>[2x]MSDVAETLDPLRLPLQGERLIEASAGTGKTFTIAALYLRLLLGLGGSAAFPRPLTVEELLVVTFTEAATAELRGRIRSNIHELRIACLRETTDNPLYERLLEEIDDKAQAAQWLLLAERQMDEAAVFTIHGFCQRMLNLNAFESGMLFEQQLIEDESLLRYQACADFWRRHCYPLPREIAQVVFETWKGPQALLRDINRYLQGEAPVIKAPPPDDETLASRHAQIVARIDTVKQQWRDAVGELDALIESSGIDRRKFNRSNQAKWIDKISAWAEEETNSYQLPESLEKFSQRFLEDRTKAGGETPRHPLFEAIDQLLAEPLSIRDLVITRALAEIRETVAREKRRRGELGFDDMLSRLDSALRSESGEVLAAAIRTRFPVAMIDEFQDTDPQQYRIFRRIWHHQPETALLLIGDPKQAIYAFRGADIFTYMKARSEVHAHYTLDTNWRSAPGMVNSVNKLFSQTDDAFMFREIPFIPVKSAGKNQALRFVFKGETQPAMKMWLMEGESCGVGDYQSTMAQVCAAQIRDWLQAGQRGEALLMNGDDARPVRASDISVLVRSRQEAAQVRDALTLLEIPSVYLSNRDSVFETLEAQEMLWLLQAVMTPERENTLRSALATSMMGLNALDIETLNNDEHAWDVVVEEFDGYRQIWRKRGVMPMLRALMSARNIAENLLATAGGERRLTDILHISELLQEAGTQLESEHALVRWLSQHILEPDSNASSQQMRLESDKHLVQIVTIHKSKGLEYPLVWLPFITNFRVQEQAFYHDRHSFEAVLDLNAAPESVDLAEAERLAEDLRLLYVALTRSVWHCSLGVAPLVRRRGDKKGDTDVHQSALGRLLQKGEPQDAAGLRTCIEALCDDDIAWQTAQ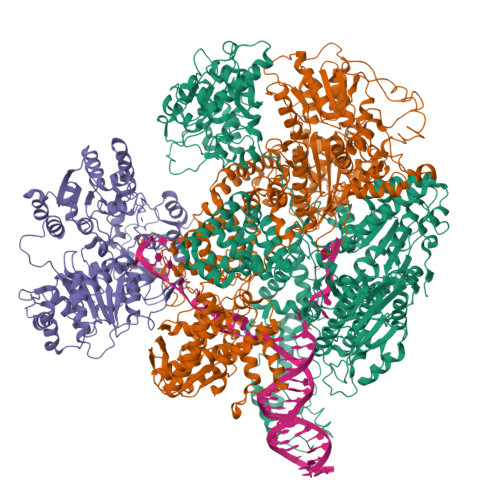TGDNQPWQVNDVSTAELNAKTLQRLPGDNWRVTSYSGLQQRGHGIAQDLMPRLDVDAAGVASVVEEPTLTPHQFPRGASPGTFLHSLFEDLDFTQPVDPNWVREKLELGGFESQWEPVLTEWITAVLQAPLNETGVSLSQLSARNKQVEMEFYLPISEPLIASQLDTLIRQFDPLSAGCPPLEFMQVRGMLKGFIDLVFRHEGRYYLLDYKSNWLGEDSSAYTQQAMAAAMQAHRYDLQYQLYTLALHRYLRHRIADYDYEHHFGGVIYLFLRGVDKEHPQQGIYTTRPNAGLIALMDEMFAGMTLEEA;>[2x]MLRVYHSNRLDVLEALMEFIVERERLDDPFEPEMILVQSTGMAQWLQMTLSQKFGIAANIDFPLPASFIWDMFVRVLPEIPKESAFNKQSMSWKLMTLLPQLLEREDFTLLRHYLTDDSDKRKLFQLSSKAADLFDQYLVYRPDWLAQWETGHLVEGLGEAQAWQAPLWKALVEYTHQLGQPRWHRANLYQRFIETLESATTCPPGLPSRVFICGISALPPVYLQALQALGKHIEIHLLFTNPCRYYWGDIKDPAYLAKLLTRQRRHSFEDRELPLFRDSENAGQLFNSDGEQDVGNPLLASWGKLGRDYIYLLSDLESSQELDAFVDVTPDNLLHNIQSDILELENRAVAGVNIEEFSRSDNKRPLDPLDSSITFHVCHSPQREVEVLHDRLLAMLEEDPTLTPRDIIVMVADIDSYSPFIQAVFGSAPADRYLPYAISDRRARQSHPVLEAFISLLSLPDSRFVSEDVLALLDVPVLAARFDITEEGLRYLRQWVNESGIRWGIDDDNVRELELPATGQHTWRFGLTRMLLGYAMESAQGEWQSVLPYDESSGLIAELVGHLASLLMQLNIWRRGLAQERPLEEWLPVCRDMLNAFFLPDAETEAAMTLIEQQWQAIIAEGLGAQYGDAVPLSLLRDELAQRLDQERISQRFLAGPVNICTLMPMRSIPFKVVCLLGMNDGVYPRQLAPLGFDLMSQKPKRGDRSRRDDDRYLFLEALISAQQKLYISYIGRSIQDNSERFPSVLVQELIDYIGQSHYLPGDEALNCDESEARVKAHLTCLHTRMPFDPQNYQPGERQSYAREWLPAASQAGKAHSEFVQPLPFTLPETVPLETLQRFWAHPVRAFFQMRLQVNFRTEDSEIPDTEPFILEGLSRYQINQQLLNALVEQDDAERLFRRFRAAGDLPYGAFGEIFWETQCQEMQQLADRVIACRQPGQSMEIDLACNGVQITGWLPQVQPDGLLRWRPSLLSVAQGMQLWLEHLVYCASGGNGESRLFLRKDGEWRFPPLAAEQALHYLSQLIEGYREGMSAPLLVLPESGGAWLKTCYDAQNDAMLDDDSTLQKARTKFLQAYEGNMMVRGEGDDIWYQRLWRQLTPETMEAIVEQSQRFLLPLFRFNQS;>[2x]MKLQKQLLEAVEHKQLRPLDVQFALTVAGDEHPAVTLAAALLSHDAGEGHVCLPLSRLENNEASHPLLATCVSEIGELQNWEECLLASQAVSRGDEPTPMILCGDRLYLNRMWCNERTVARFFNEVNHAIEVDEALLAQTLDKLFPVSDEINWQKVAAAVALTRRISVISGGPGTGKTTTVAKLLAALIQMADGERCRIRLAAPTGKAAARLTESLGKALRQLPLTDEQKKRIPEDASTLHRLLGAQPGSQRLRHHAGNPLHLDVLVVDEASMIDLPMMSRLIDALPDHARVIFLGDRDQLASVEAGAVLGDICAYANAGFTAERARQLSRLTGTHVPAGTGTEAASLRDSLCLLQKSYRFGSDSGIGQLAAAINRGDKTAVKTVFQQDFTDIEKRLLQSGEDYIAMLEEALAGYGRYLDLLQARAEPDLIIQAFNEYQLLCALREGPFGVAGLNERIEQFMQQKRKIHRHPHSRWYEGRPVMIARNDSALGLFNGDIGIALDRGQGTRVWFAMPDGNIKSVQPSRLPEHETTWAMTVHKSQGSEFDHAALILPSQRTPVVTRELVYTAVTRARRRLSLYADERILSAAIATRTERRSGLAALFSSRE>[6x]LTAKKRPSVVYLHNAECTGCSESVLRTVDPYVDELILDVISMDYHETLMAGAGHAVEEALHEAIKGDFVCVIEGGIPMGDGGYWGKVGGRNMYDICAEVAPKAKAVIAIGTCATYGGVQAAKPNPTGTVGVNEALGKLGVKAINIAGCPPNPMNFVGTVVHLLTKGMPELDKQGRPVMFFGETVHDN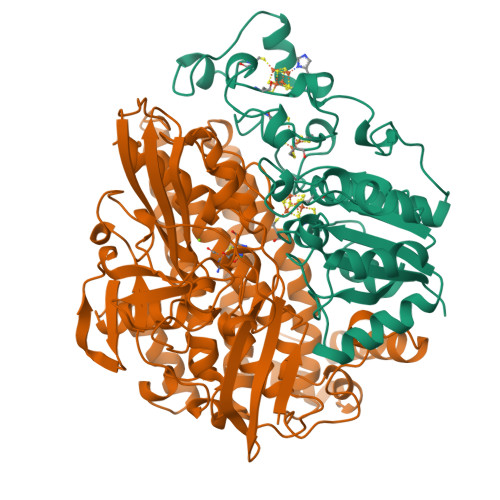CPRLKHFEAGEFATSFGSPEAKKGYCLYELGCKGPDTYNNCPKQLFNQVNWPVQAGHPCIACSEPNFWDLYSPFYSA;>MSEMQGNKIVVDPITRIEGHLRIEVEVEGGKIKNAWSMSTLFRGLEMILKGRDPRDAQHFTQRACGVCTYVHALASVRAVDNCVGVKIPENATLMRNLTMGAQYMHDHLVHFYHLHALDWVNVANALNADPAKAARLANDLSPKKTTTESLKAVQAKVKALVESGQLGIFTNAYFLGGHPAYVLPAEVDLIATAHYLEALRVQVKAARAMAIFGAKNPHTQFTVVGGCTNYDSLRPERIAEFRKLYKEVREFIEQVYITDLLAVAGFYKNWAGIGKTSNFLTCGEFPTDEYDLNSRYTPQGVIWGNDLSKVDDFNPDLIEEHVKYSWYEGAGAHHPYKGVTKPKWTEFHGEDRYSWMKAPRYKGEAFEVGPLASVLVAYAKKHEPTVKAVDLVLKTLGVGPEALFSTLGRTAARGIQCLTAAQEVEVWLDKLEANVKAGKDDLYTDWQYPTESQGVGFVNAPRGMLSHWIVQRGGKIENFQLVVPSTWNLGPRCAEGKLSAVEQALIGTPIADPKRPVEILRTVHSYDPCIACGVH[6x]> MTADELVFFVNGKKVVEKNADPETTLLAYLRRKLGLRGTKLGCGEGGCGACTVMLSKYDRLQDKIIHFSANACLAPICTLHHVAVTTVEGIGSTKTRLHPVQERIAKSHGSQCGFCTPGIVMSMYTLLRNQPEPTVEEIEDAFQGNLCRCTGYRPILQGFRTFAKNGGCCGGNGNNPNCCMNQKKDHTVTLSPSLFNPEEFMPLDPTQEPIFPPELLRL;> KDVPPKQLRFEGERVTWIQASTLKELLDLKAQHPEAKLVVGNTEIGIEMKFKNQLFPMIICPAWIPELNAVEHGPEGISFGAACALSSVEKTLLEAVAKLPTQKTEVFRGVLEQLRWFAGKQVKSVASLGGNIITASPISDLNPVFMASGTKLTIVSRGTRRTVPMDHTFFPSYRKTLLGPEEILLSIEIPYSREDEFFSAFKQASRREDDIAKVTCGMRVLFQPGSMQVKELALCYGGMADRTISALKTTQKQLSKFWNEKLLQDVCAGLAEELSLSPDAPGGMIEFRRTLTLSFFFKFYLTVLKKLGKDSKDKCGKLDPTYTSATLLFQKHPPANIQLFQEVPNGQSK;> EDTVGRPLPHLAAAMQASGEAVYCDDIPRYENELFLRLVTSTRAHAKIKSIDVSEAQKVPGFVCFLSADDIPGSNETGLFNDETVFAKDTVTCVGHIIGAVVADTPEHAERAAHVVKVTYEDLPAIITIEDAIKNNSFYGSELKIEKGDLKKGFSEADNVVSGELYIGGQDHFYLETHCTIAIPKGEEGEMELFVSTQNAMKTQSFVAKMLGVPVNRILVRVKRMGGGFGGKETRS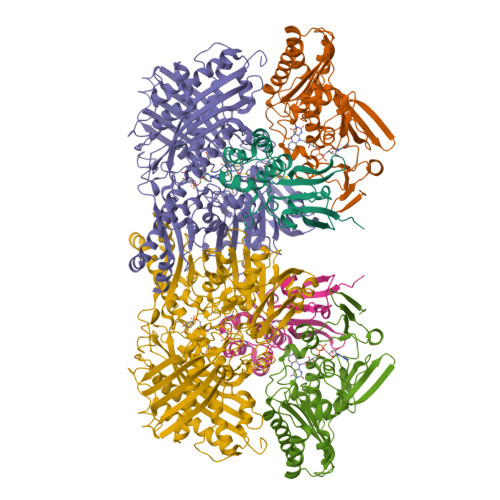TLVSVAVALAAYKTGHPVRCMLDRNEDMLITGGRHPFLARYKVGFMKTGTIVALEVDHYSNAGNSRDLSHSIMERALFHMDNCYKIPNIRGTGRLCKTNLSSNTAFRGFGGPQALFIAENWMSEVAVTCGLPAEEVRWKNMYKEGDLTHFNQRLEGFSVPRCWDECLKSSQYYARKSEVDKFNKENCWKKRGLCIIPTKFGISFTVPFLNQAGALIHVYTDGSVLVSHGGTEMGQGLHTKMVQVASKALKIPISKIYISETSTNTVPNSSPTAASVSTDIYGQAVYEACQTILKRLEPFKKKNPDGSWEDWVMAAYQDRVSLSTTGFYRTPNLGYSFETNSGNAFHYFTYGVACSEVEIDCLTGDHKNLRTDIVMDVGSSLNPAIDIGQVEGAFVQGLGLFTLEELHYSPEGSLHTRGPSTYKIPAFGSIPTEFRVSLLRDCPNKKAIYASKAVGEPPLFLGASVFFAIKDAIRAARAQHTNNNTKELFRLDSPATPEKIRNACVDKFTTLCVTGAPGNCKPWSLRV>[2x]MTQLTREQVLELFHQRSSTRYYDPTKKISDEDFECILECGRLSPSSVGSEPWKFLVIQNKTLREKMKPFSWGMINQLDNCSHLVVILAKKNARYDSPFFVDVMARKGLNAEQ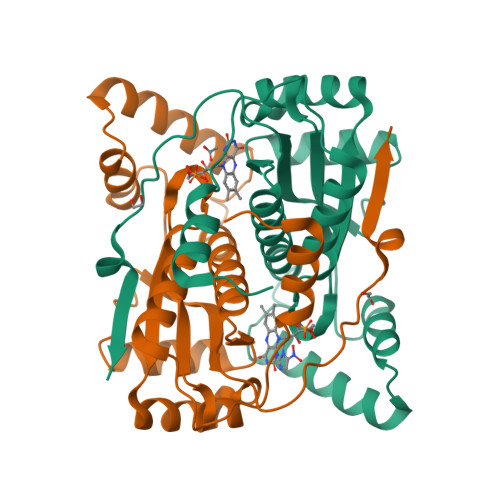QQAALTKYKALQEEDMKLLENDRTLFDWCSKQTYIALANMLTGASALGIDSCPIEGFHYDKMNECLAEEGLFDPQEYAVSVAATFGYRSRDIAKKSRKGLDEVVKWVGKLAAALEHHHHHH> APVRSLNCTLRDSQQKSLVMSGPYELKALHLQGQDMEQQVVWSMSFV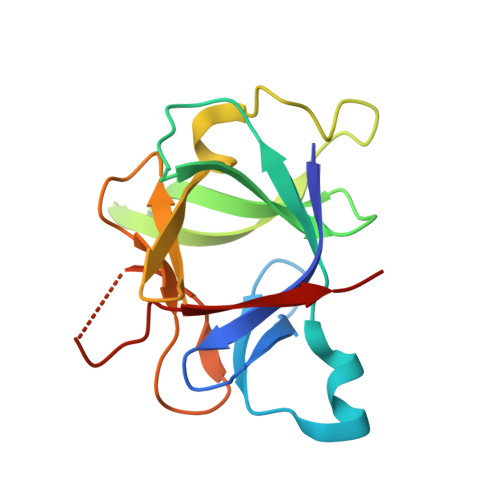QGEESNDKIPVALGLKEKNLYLSCVLKDDKPTLQLESVDPKNYPKKKMEKRFVFNKIEINNKLEFESAQFPNFYISTSQAENMPVFLGGTKGGQDITDFTMQFVSS> GDDDDDVKNEVVVSFENLLTEENSQFIADGTPNNQAFQETDFKDPKNLINFNHYYADWGSGYSFAGFSYMNITDNQTANSPAPITGKAKIGSVYIGVDSTDGEYGTPAILTILDTNYKLKGTWIANSTWAYMGMIQGDGYARAFKAGDWYKVTATGYDEAGNETGKAEILLANYKTDNDLPVKEWIWFDLTPLQNAVKVKFIPDSSDKNEYGMNTASYFCLDGITL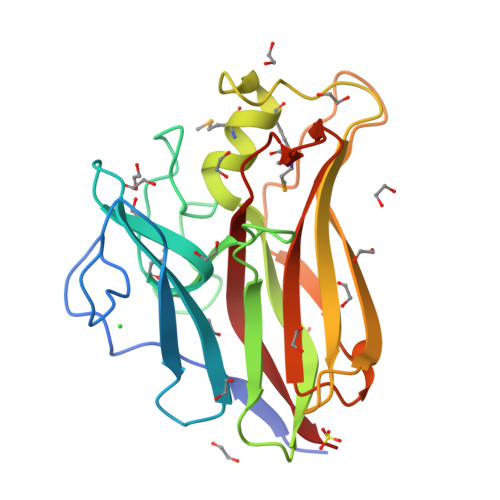IEK> VGVEDVGRFRLFDRHRLVELLPEGLAGELSRDVEMIPSATSPIGVMLRKATLELQMQLELFARVHAKSSADTRGETPLPRKRKETRKDGERDAREKKKDEGKDKDGGVGGRGLEEIGSRRSEDEWRERLSELRPFDARLAAVQRGFLLDGHRGVGKSCVLNYLIPWARENNWLVVYEPLPSRYAREIGDIKRSSAGVYIQSSFSQEFLERLGRFNRRLLEELPVARRCYGQAALDGVHRLYAERSYHSLLEKALEKDLDEIREQRDEELKRGSPHSGKDADLLDSQLREEILLARERLALWHTYRREVSIPSMKSRLPNPASVWEIAEFGLQNEAFATQALYEVWEQLKKQTQLNVLIAVDEWNECFPVSEYVSMRYEGTRFNGHIPAFHLSTPRLLSRFDDAQQFQRGLKICATSWRRSNRRDYRPDLLGVRQEEIRTVRNFSPLEFANFVAYYHKKKILHEFPREKLDYFYMLSGGNGFQARRLLASLYGG;> SSDSALISGAIVRAFNPERMKVFMHNGCEWLWQAEGTGTRKRAAAHVIIRRGTGQVRVNNDEDLYVRWPFYYNRMDVLQPFFLTGTAGIYDLFIHVRGGGSSGQAGAVRLAVGRALVSACPACARLLEEDMVLYEDTRQRMPKMPGRMKARKMRTW;> ALSAYSLRSLIVTYNSRNRSSMNATIENLKNALRWTSPSESSSPSSAPSSAPSSAPSSSWSPPWPVPRRVGRRQWRVTYLKSPFKYKYALRHYVFEDHRYAFAFYDVNSVQEVVSAALGAMAGETCCSCRFSWRFAGRPPVSLPTPPRLVPSSRAASLLSSRSSSEDGEVSREPVEGGEKTSGVKKAPHLATVLRGHCPTDKEFIRRALEEEQAVERIRKKLDKKQLQWFPGKTPWAP;> LNPPPIAFPSFNRRCQKDWLARRAFAENEVNGRIYKNVYQNLGFKGPIPILNKVGQYRIRMRCISGGYSRGIFRFTRMARMGMLQLAREGWLKKYGYRPGLF;> ARRVGGIGRRCFLTLHCSACSFFFQTSDAIKLILTQQHHILRKKGETRFLSGASGDAVHLESVGASNEAQGNRPSSSSSPSSSGGTRDKGVSRRVVAAAASSAASKFSLLPLADASLLLKRRGALVLRSLHGDPLVGSRRQRGEFAPQAPTAEMAKMLNKSCVPCPRCKREGRWEEG;> YITSANFSEPVELLSLAEDLHKAEIYTQTTEKLEKQWPAAGGVAKGIQGDQFFDVMAAAVREDLQDQSRPVLVNELTDHENPYCMKREALRRLVLHACTRNCLDETLTDTLLDRRADLQRLRSKARLPPEVLEPLAAFVGITRFSFDRRARLNQKVTAVQHALRQISLDGVNTAELAEGQDEPTMDAEKVEAVLSVLPENFPSDALHPHHPFRNHFGFESSVPYGVVGSISMGKGRKKIEKELARLRYPTLQRVAHSLPKDLKYRESVAHAIRVLERSRGWDFESKVKAVNALVEVWNRLAPGRTYEKILNHAFPVFRGRGMVKKTRSRAAVFNKGLKYIRSLTTQKPLHARLQ;> PAERLHSLFARADVLAHLLHSRLALPLLYPLNSGGALTNPLNSAASPDSPAALNSIATSRWKREEVMSALATVTPLVLAATSVSRFLKTAHALSYFA;> PEAPQPPAGLHWSWWELYVKGVNPEYPPRQRMFAFLTAQGVDVLEMEIREIEDVTRWLEMSNVYGEKFPRFPYDVTFQDKIEALKEKYPL;> AFRYRREGQFTKFRVHFDRSGFRPYIDELKWEIMDWHYKRAMGPQMKKTLMSYQEGSEKLQYMHDLIALGTAKAKFPHATKRFFFVPALPVTIPYRRSSNPFCLLSANKTGWLQWSPKQRVPFPQPLGKRKVGGTDPQPPVFPK;> LQELESFVGSALRTYRLLRPHALPFYKEDSLLSMQSKLNEATLKHSPLVHDLVELKKRNLSVPSDLLPPDFNALQFSLPVVSARGFLLALSAAANSVAEDLEFLCRRLSVPNLPHPTHPFRLKLLLDALFESFKLRKDPHYAHDWAQRNWPRLQAAMPEPLSELSADSVGLWLKAHLERVIENQRGRHADGRGRLLAQKFPLKSDEEDLYSLADDFIFDHEIVDEQFCDERLSQFPIDKAGELFRRVADFFGLTKGPQPAVNDAVVAQFQNLVYTLDEIGLSNWMKMDTREIEEFLPEGDPPSFAASQQDLDAARLLLKAAARGKANLLDFEALDPYKLLHGFDFKTVQEELATLPPNPFLTDADIDELFDITTAAVSMNQSEVAPSASLRNFKAKFGRTPLEALLDSEEKFLTSAGPVDWLKDEDENGEAFVSWRWKRPA;> EEDDSVYRQFACMRRVREEPRLRTALESFKVASKNATKTRGRAWSVYEGWPPRSRVRVGDEYSKVGPLQRRAFVFNRVDGTGRRREPTLAFCCGNKPVLLLSEAEFEALVKKLPWIKHEMAEFKKLL;> RQAKKQTKLAAKNARKMKESKGLLLEGKKTALCMNLMQNTGIAWYRSLQVCKHLEMHRRAPVPRVTAGFREKVTQAVAVVKLG;> FSSLRLSQKDARGSGYLPAQRFLSLLKASPEEYRSLLREATQAKIVDPAFLRVASQRFFALSDRFYPPEILDILSDFASFPYSDEALLAAVAGRLEDQLVEPSPKRLAALLSLSARLGLCHPSIRDPLTKHIEEKMYAFDAALLDSLCRTVGSLLSPRLPLLDGLATQAQLLASDLRAGEQSLETGDEVAQRRYIALLFRCLEGLSRQRYSQSALVDACVACAEQHGQAFPLHDTLRAVAAARRLDLAGIEEPLRRSDMADKVNRATDRGDQLLALLRHLDLLRLRDSQLLQKVSEAVELHSQKAAFLATQLPEALLHLTRLAPADLRLPVALLSQPSLLAMAPRLSAAQLQQLLSASALVLFQHIQRREGGQGGDPLIAREAEALAKTVERFLDLLKPQFLSLNLRDRRALKEAASLFLVEAKGAAKSSAASPQFALAPKTVDFCCFLEEADVAPPLPLAPSGGVDFQSVGLVEACSRLVLCADARFSETRNSARGASEGDTKKGDSEKTSLPQTAGRDMEAAAKQRALLFVSPRDAFADARRSRGETVSKSSKAKEREETTTCKLGGVSTDLPVSITPQAASSLLLTQLALIRRGILRHEIQTCIPPP;> CMNKKNRLALRKRRRRMGERVSLRYR;> TRGFRWDLCQRGRRRWVHINYPPRNRSTVQMLDESHEKLVFVCNGYIDRLDPRLLPERLRKRLERNRKAALTRFDGKLPWGQAVESAIKRIHTPCLAFAQAHSHHLLEAFSMAEVLEIEKLIPEIREAFKASKAKLAEQEAQDKFTRHVSVDLVDLKEDPVSFPFTLK;> KKKRGKKEKVILNAEQVATKTRLPPIRLEDRITPEPPATVARNIRSQISRAVAGWKTKRMFTYRNKYRLRRLVGMTHDIDSDDEFAQANARTRETNASTSKVSSSGCSTEKAEGVNGSTMGRRNRPSFAGRTFVTPLTKLQHQAALPRSPLHARFDFPHTVHYDVFWGPPQVEEEPNKSGCWVSFRVADLKLSDSQEQRLLDILGPERYDEQTGVVCLEADVFPQLNHNAAYLGDILQQLMREVKK;> LLDTGEIVPGAFASVKKVGDFPLLPLSLLLSRLKERRQELLRDWQVHAVRQAAVREPLAEATRENDGGAGPRAVEAFAREEERIQRKIKILELLACGGLEENASSQGAIGDAKRIAFLAHADAVNLLLLLAAEAETLARPGEREETEGKEGSSAVGEISKQEERQLWRLKCEGNEEKWNLCISRLKELALDHEDSFLVFYAMCSTNRFDAVLLPALLERLEASFFSSQALSKPLFHPIFEVWDPPCESFAALINVLPLSAKAVVVTADRRSERERRENEGWLAPPEAPPLVLPNWQTMHPVDMEAWEKKQRRVVRTRHVKAKIIRQADGRKLAATMALHGRQAIHRDAAVSSLVSVAAMCASNSQRALRGELLPETLNLLAAELLGRSADALSPHLLSLSFLLSQSSVSLTERLFLHLEAVLRGWLEENGFVEKKQTENVDGESKELCTETASEKRRKASEEQLRNLPPGLNVFGLVQSSPSSSDALLASGERSETSKSADTESALWESRVLAALLSSFLRVDDYRPSLDFVLLLSDALRNSLRRTAVLSSASESSAPLAIHEKDVLSLKETGALLSSFATSGYAVPPSLMACLVEHFLYDVDLFLTSSPLSPFASSPSSSSSSAEEAEQLSQSFFCSSRGRATPGDCATLLHSLASPSPLSSERLAAADKAGEQKTANLEKLRFEAMTQAWRLVAPVLHLLQPPCKLLILNSLQTAHAPPDVSSTAFFQRSLETFLRDNPDVDSSLLGSLFGTQGR;> RQEFFWPEKARRTRVPLYQNSRPNLVYDQRFRRFMCMWYANGVQVFRPFSCRGRRGGRGKEGLPDGLGIGRGSGTWERARAKAVVLLKQLQRQGHLDRLAKPDVTRSGVRGVYFDTEEKLWVATWNEHGLRRFKAFPTMEMGFDAAYQAAVAVRRQKLRENYIFSMQRNR;> TAPRVVRDRDETNFHEMLGKFRFDLQGSFKENGDMLRDSLLQVGRDLFLVGWVKCRSRFATGHIQGDVHALSYMRRYLEKHVDESVSSVRFYEENFGMPLLEYERLSAVNDFRAPGKKQQH;> MRRLASPSLRRLQEGQTPHSMRKSAVADARKKIFGYACGMPGEEQWVRPLQGRQMMKWYWPSKYMLQDVQMAQYFQMQAMRFAPRPAHVSLTTLSATMEQCWKKRDAVRAFFQSIDEKVLRENPTLQDLYGLYRTLCPDDPLRTPVDPALWRDPGFTWQHTADQRIVSSSTNREQQGDPSEPAMATRRVAQEQATDKRHISPANINDDVAALLFSRTEQSGAIRNVCAASPYLHGGKNNRSRDRFHNGAREANSSEEDSLEQPKSLILDTESRGTALSRSRTQECLLALSALAETGLGQSASELIQQPVVLRVDIGLGDREPVQDTTAFRKKQEQSRRTLQAALDHDERLARYHGAKHRFFDPLFRRRRLSFLDRFARERIKGEKARQLGAQLYVKHPDQKPVWP

Our study reveals how Toxoplasma gondii assembles over 40 mt-rRNA fragments using exclusively nuclear-encoded mitoribosomal proteins and three lineage-specific families of RNA-binding proteins. Cryo-EM analysis of the mitoribosome structure demonstrates how these AP2 proteins function as RNA binders to maintain mitoribosome integrity. The mitoribosome is also decorated with members of lineage-specific RNA-binding proteins belonging to RAP (RNA-binding domain abundant in Apicomplexa) proteins and HPR (heptatricopeptide repeat) families, highlighting the unique adaptations of these parasites. Our results reveal the structure and composition of the most fragmented rRNA mitoribosome to date.

The LSU was resolved to 2.89 Å, and the entire mitoribosome was locally refined to three bodies, the SSU head, the SSU body and the LSU, at resolutions of 3.6 Å, 3.29 Å and 3.11 Å, respectively. The first striking feature is the relative size of the SSU compared to the LSU, as the former appears substantially larger with an elongated oval-shaped head. The SSU harbors two particularly protein-rich regions, on the top of the head and the bottom (foot) of the body. On the top of the head, a cluster of mainly three large proteins (mS29, mS139 and mS141) form a tight domain around two short unassigned leftover rRNA fragments (ulr22 and ulr23). Interestingly, the universally conserved uS3m at the entrance of the mRNA binding channel is absent in the T. gondii mitoribosome and is instead replaced by the C-terminal and N-terminal tails of mS151 and mS148. Finally, one must highlight the absence of the conserved uS7m at the exit of the mRNA channel in T. gondii, a position that seems to partially overlap with mtAP2-1. Also, uS5m is substantially enlarged in this mitoribosome, as it has acquired a large SSU-head domain and N-terminal and C-terminal extensions on the SSU body. As anticipated, mtAP2-1 on the SSU is located at the head-to-body junction near the platform. Specifically, mtAP2-1 interacts mainly with fragments SSUB and SSUD with its first AP2 domain binding directly to the 3’ end of SSUD and interacting minorly with SSUB, mostly via arginine residues with the RNA backbone.> MAHHHHHHMEQKISVALKEIKRGANEIIGLEYIEKLVRKYYETNERFIVKAGFDPTAPDLHLGHTVLIQKLALLQQYGARVKFLIGDFTAMIGDPTGKNETRKPLNREQVLENAKTYEEQIYKILDQKHTEVCFNSTWLDALGAKGMIELCAKFSVARM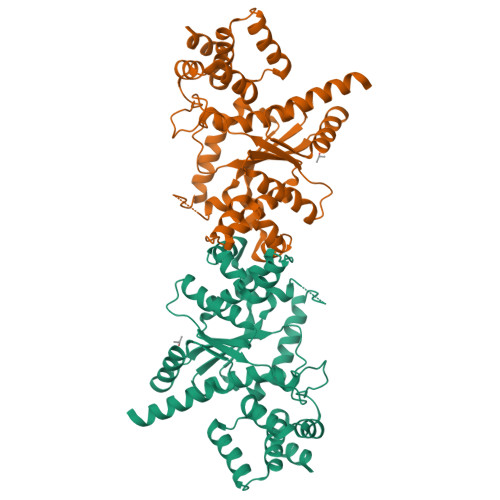LERDDFAKRHKENRPISIVEFLYPLLQGYDSVAMGADIELGGNDQKFNLLVGRFLQRAYGLNKEQSIITMPLLEGLDGVQKMSKSLGNYVGITEEPNAMFGKIMSVSDDLMWRYYTLLSAKTLEEIEDLKHGILNQTLHPKAVKEDLAGEIVARYYDNDQAFKAKEQFSKVFSANLLPEILSESDFDEGVGILDVLKQIGFCPSTSQARRDIQGGGVKINQEVIKDESYRFVKGNYVIQLGKKRFMKLNIN> KNPKSDKFKVKRFHHIEFWCGDATNVARRFSWGLGMRFSAKSDLSTGNMVHASYLLTSGDLRFLFTAPYSPSLSAGEIKPTTTASIPSFDHGSCRSFFSSHGLGVRAVAIEVEDAESAFSISVANGAIPSSPPIVLNEAVTIAEVKLYGDVVLRYVSYKAEDTEKSEFLPGFERVEDASSFPLDYGIRRLDHAVGNVPELGPALTYVAGFTGFHQFAEFTADDVGTAESGLNSAVLASNDEMVLLPINEPVHGTKRKSQIQTYLEHNEGAGLQHLALMSEDIFR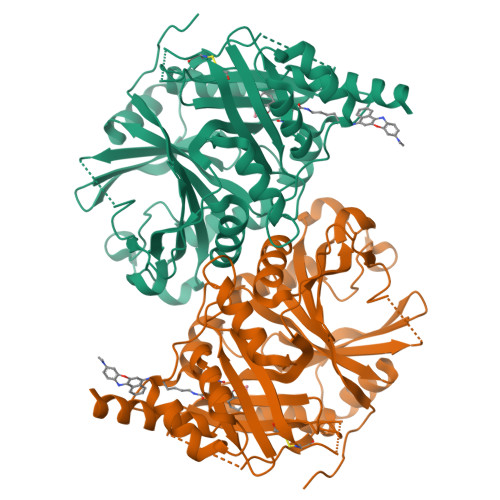TLREMRKRSSIGGFDFMPSPPPTYYQNLKKRVGDVLSDDQIKECEELGILVDRDDQGTLLQIFTKPLGDRPTIFIEIIQRVGCMMKDEEGKAYQSGGCGGFGKGNFSELFKSIEEYEKTL> VTLTLALAVAFGIAAISPLLARTMGRDAGWPLAAMLGGLALYIWFAIPVDTVASVEWMPALGVELRLSLDPLARVFTMIVLGIGAVVMAYSSRYLGRGSGHGGYYGLMTLFAASMLGLVLADDVVVLFVAWEFTTLCSFFLITLAGPKGTQPAVRTLLVTVAGGLCLLTAAALMVVRTGTTVLSEILVDPVWSADPAFAAVIAVLIAMAAFTKSAQFPFQAWLPDAMVAATPVSAYLHAAAMVKAGIYLLLRFSEALHDVPVWNLLLITCGMTTAVLGAVFAMQRDDLKELLAYSTISQLGFLVATIGVGTPAAMVAAIIHTIAHALFKSSLFMFVGVVDHQTGTRAMSGLPRLYRIMPGTAIGVGLAAASMAGLPPLLGFVSKEWMFKSMLDAPGGAWAGPALGALAVFAATFTFAYSARFLLGGFVTHGPPAGPGPEPVHSTPETIEAPRASFFLPAALPAVLGLVLGLTGFLLEPAVAAAARASIGEGYEADFGLWHGFAPELFMSMIVITLGIVLVVVRHPVDRFLDRELAPITGVATVDALRRWAIAGGARVGDVTRTDRISRHVWAVLLVLVALAAVGVVAVRPEPEVGSPVRAEDWIVVVLLVVGTAAMVISRSRLGAVANVGIVGFAMALWFFTLGAVDVALTQLLVEVLTVVVIVLVLQRLPRAFHTVSRSRTLVSAAVAIVVGLASGAAVWAMTGRRELSDVGRYFLDNAEQDTGGINVVNTVLVDYRALDTLGELTVLGVAGLAVILALHARRALPRRDVPLAVHADSPLLSAQDNGVFLRTFARILGPLIVLLSLYFLVRGHNAPGGGFNSALIGGAGIAIYYLRAPSDKAARIRVPYVAVIAAGVIIGVVTGLAGFVDGSFLLPLHAYLGDVHLTTALIFDVGVYLAVLGVIMAAIDKLGG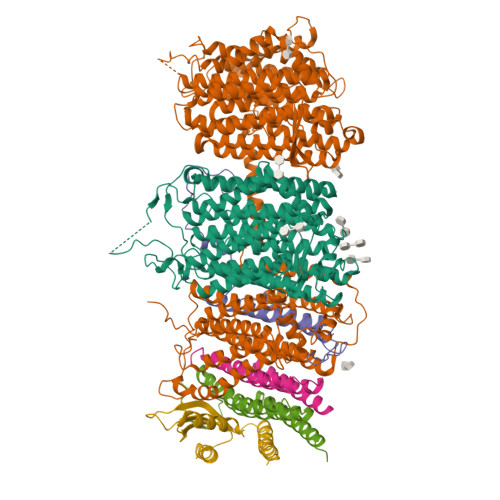DDRSDEPAVPPPPPTGPGAEATAPAATEDADRVIDVTDNREVQA;> MTLAISVGVLMAGFVFLVLQRGMVRVILGFILLSHAAHLTLMAAGGASRREAPLVSDPDPALTSDGLPQAFVLTAIVIAFAITIYLLVLAVIGGDDDDTDIGDLDPLDLLPETPGGAHPEDPEPDEPSTHDAEGVHR;> MTLESALTLFVAVPLLTAGVLVAVASRTRLILTVLFAVLGTQLAAAVATVPWVSDGSVVVHQVALWAPGVSIPFVLDMFSALMLTVTSLLTLTCAAFAVAAGEAYKRFYPPLVLLVTAGVNGALLTGDLFNFFVFVEVMLLPSYGLMMITRSGRASVVGVAASRLYISVNLLASTILLIGVALIYGVTGTVNIAQLHGAASEDTAVAVATALVLFALAIKAAVVPVHGWLARAYPKMSPAVTAMFSGLHTKIAIYAIYRIYAVIFDGDSRYLWVGVVVFSATMLIGVLGAVGEAAPRSILAFHMVSQIGYILLGVALFGPIGLTAGIFYLLHHMIVKAALFLAIGAIEVRYGPRRLGQLSGLAKTEPLVAVAFFASAMSLAGIPPFSGFVAKLSLIIAALDAGQIAAAAVAVVVSILTLLSMLKIWTGIFLGEPTPTDSRTLPEGLDPAHSEATGIPDGRDVDGRHRDGVEITGAAAGATPTDTMAPASTTATATATDTVTETASVADTAEAGSPDPDMVPPGRRIGLALAAPALALSVVTLALGLGGQLLLELSGTAAANLYDPTTYIQAVLG;> MTSTLTWPLRIAWFLLWFFWQQTTTSAKVVRDAFLPHASITPGFVRFPTRCRSELEVTMLSSLITLTPGTLTLGAHHPGEGEDWEIVVHGMYFPDPDDLTASLHDLENHMLRAIRREGLTR;> MIVVDIAIVLVAIAAVLSSYRMIRGPHAGDRAIAADLLFFAFIALLALVGVRVDSPFVYDLVLVATLVGLVSALSLARLMSGGRR;> MSWELVATVLGSVSVLVGAVVFLGGAIGLLRFPDLYVRSSAIGAAAGLGLVFVIAGAFLLHPTWEAAPKVAVAAILQFASSAIGAMYIARAGFLSGAAPTTATRYSQIEFTTGPPTDSTEVTRDD> SKGFFVDTTRCTACRGCQVACKQWHGNPATPTENTGFHQNPPDFNFHTYKLVRMHEQEIDGRIDWLFFPDQCRHCIAPPCKATADMEDESAIIHDDATGCVLFTPKTKDLEDYESVISACPYDVPRKVAESNQMAKCDMCIDRITNGLRPACVTSCPTGAMNFGDLSEMEAMASARLAEIKAAYSDAKLCDPDDVRVIFLTAHNPKLY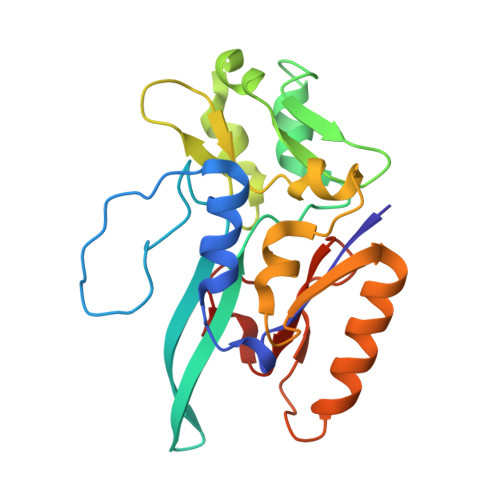HEYAVA> GKSASMAVEEIASRKDISLRDMQISAILKMLFLNKDLNNNDNITTITDDIFNQQEIIWKVLILDIKSTATISSVLRVNDLLKAGITVHSLIKQDRSPLPDVPAIYFVSPTKENIDIIVNDLKSDKYSEFYINFTSSLPRNLLEDLAQQVSITGKSDKIKQVYDQYLDFIVTEPELFSLEISNAYLTLNDPKTTEEEITGLCANIADGLFNTVLTINSIPIIRAAKGGPAEIIAEKLGTKLRDFVINTNSSSTSTLQGNDSLERGVLIILDRNIDFASMFSHSWIYQCMVFDIFKLSRNTVTIPLESKENGTDNTTAKPLATKKYDIEPNDFFWMENSHLPFPEAAENVEAALNTYKEEAAEITRKTGVTNISDLDPNSNNDTVQIQEVVKKLPELTAKKNTIDTHMNIF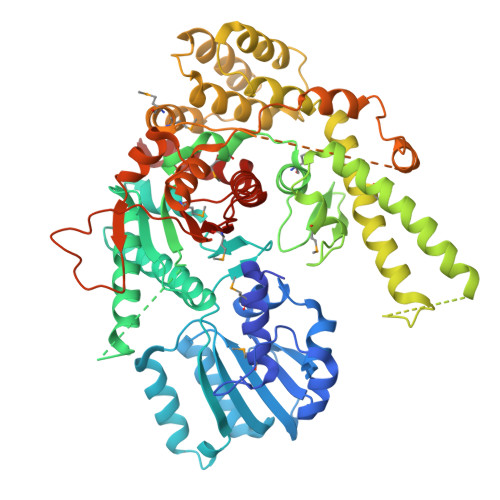AALLSQLESKSLDTFFEVEQDPGSTKTRSRFLDILKDGKTNNLEDKLRSFIVLYLTSTTGLPKDFVQNVENYFKENDYDINALKYVYKLREFMQLSNMSLQNKSLEDGSDSAFKPSNLTLSGIYGLTEGKLQGGVGSLISGIKKLLPEKKTIPITNVVDAIMDPLNSSQKNLETTDSYLYIDPKITRGSHTRKPKRQSYNKSLVFVVGGGNYLEYQNLQEWAHSQLHNPKKVMYGSTAITTPAEFLNEISRLGASNSSNNDA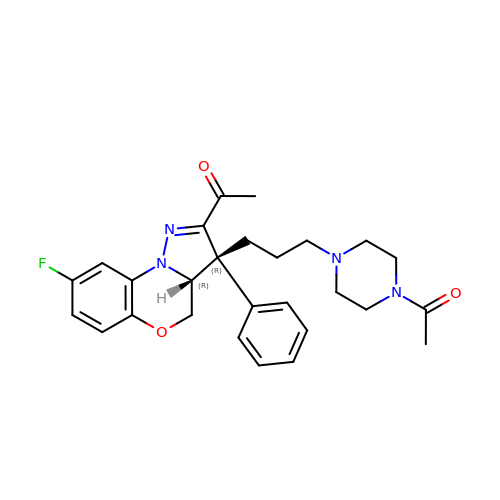1-{(3R,3AR)-3-[3-(4-ACETYLPIPERAZIN-1-YL)PROPYL]-8-FLUORO-3-PHENYL-3A,4-DIHYDRO-3H-PYRAZOLO[5,1-C][1,4]BENZOXAZIN-2-YL}ETHANONE | C27 H31 F N4 O3 | BWKAHABETZLDBG-AHKZPQOWSA-N> A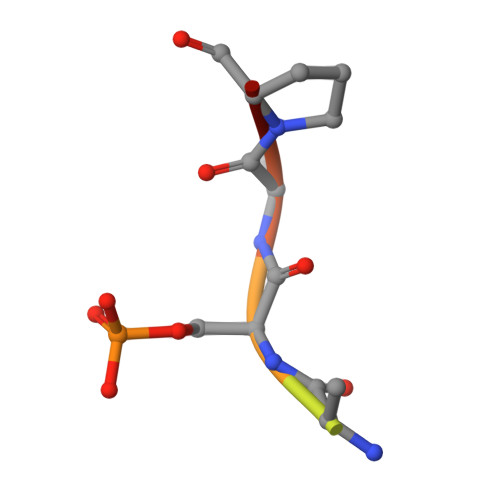RAASAPA Zinc is essential for virulence and survival and is acquired solely by the ABC transporter, AdcCB, and two Zn2+-specific cluster A-I SBPs, AdcA and AdcAII, in S. pneumoniae. Although both SBPs share this structural core, AdcA also has a C-terminal domain (residues 322 to 501; here termed AdcAC) that is structurally related to ZinT, a periplasmic protein from E. coli and Salmonella. The AdcAC domain is linked to the N-terminal cluster A-I domain of AdcA (residues 1 to 311, henceforth referred to as AdcAN) by an 11-amino-acid linking region. Collectively, our data show that the AdcAN domain is necessary and sufficient for Zn2+ acquisition, with the AdcAC domain and the His-rich loop aiding in Zn2+ recruitment during growth under Zn2+-restricted conditions.

The high-resolution crystal structure of wild-type, Zn2+-bound AdcA was determined at 1.58-Å resolution and revealed a two-domain organization with the AdcAN and AdcAC domains forming discrete globular regions, connected by an 11-amino-acid linker and each containing one Zn2+ ion. The AdcAN domain has a two-lobed organization, with the N- and C-terminal (α/β)4 lobes bisected by a cleft in which the metal binds. The binding site in AdcAN is comprised of three Nε2 atoms from His63, His140, and His204 and one Oε2 atom from Glu279. These four residues bind a single Zn2+ ion via 4-coordinate geometry, with bond distances of 1.98 to 2.08 Å. Electron density was not observed for 14 residues (120 to 133) of the His-rich loop, consistent with the predicted flexibility of this region. Intriguingly, the AdcAN domain was observed in a conformation that partially exposed the metal-binding site to bulk solvent, with the relative solvent accessibility of the metal-binding residues (His63 > His140 > His204 ≈ Glu279) remaining the same during the five independent MD simulations. The partial opening of the Zn2+-binding site of the AdcAN domain arises from the α7β6 loop having moved away from the binding site due to rigid-body rotational movements of α7 in a plane perpendicular to the helical hinge interlobe helix α5. In Zn2+-bound AdcA, interaction between the domains occurs between α12 and α15 of the AdcAC domain and α7 and the base portion of the His-rich loop (residues 109 to 117) of the AdcAN domain, with a buried surface area of ∼1,200 Å2. The most stable part of the interface involves the salt bridge between Lys368 and Asp213 and H-bonds formed by the side chain of Tyr365 with the backbone and side chain of Asp213 and the backbone of Leu212. Our structural and computational data reveal that the AdcAN domain and the AdcAC domain form a stable interaction, with the His-rich loop positioned at the interface between the two domains.

> GKLNIVTTFYPVYEFTKQVAGDTANVELLIGAGTEPHEYEPSAKAVAKIQDADTFVYENENMETWVPKLLDTLDKKKVKTIKATGDMLLLPGGEEEEGDHDHGEEGHHHEFDPHVWLSPVRAIKLVEHIRDSLSADYPDKKETFEKNAAAYIEKLQSLDKAYAEGLSQAKQKSFVTQHAAFNYLALDYGLKQVAISGLSPDAEPSAARLAELTEYVKKNKIAYIYFEENASQALANTLSKEAGVKTDVLNPLESLTEEDTKAGENYISVMEKNLKALKQTTDQEGPAIEPEKAEDTKTVQNGYFEDAAVKDRTLSDYAGNWQSVYPFLEDGTFDQVFDYKAKLTGKMTQAEYKAYYTKGYQTDVTKINITDNTMEFVQGGQSKKYTYKYVGKKILTYKKGNRGVRFLFEATDADAGQFKYVQFSDHNIAPVKAEHFHIFFGGTSQETLFEEMDNWPTYYPDNLSGQEIAQEMLAH>[8x]MTTRTTDNPWLDARVLNMAHAGGENEAPANTLYAFKRAVKLGANMLELDVQSTKDDQLVVIHNATVDQTTDGTGKVRDLTFEQVHELDAAYNFIPGRHAVPGEPPESYPLRGVRTGEKKPPPGYQPSDFAIPKL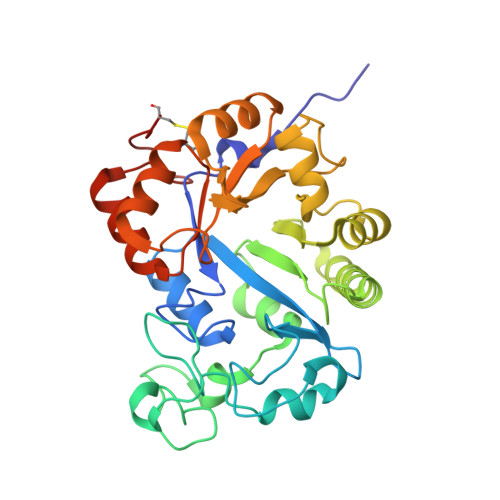ADVLEAFPRTPINIEIKGTSDADIPSFLHNAKLLARLLKKTGRTDFIVTSFNDLAVAKFHLLAPDIPIAPGMAGLAAYFLLGVKPMHGTVALQIPVRYQGLEIATPEFIRRAHADGYAVHVWFSGTAPDDEATYNRIIDSCADGLMPAYPALLERILDERGIERPGRPGVDPCGHHHHHH>[4x]MSKK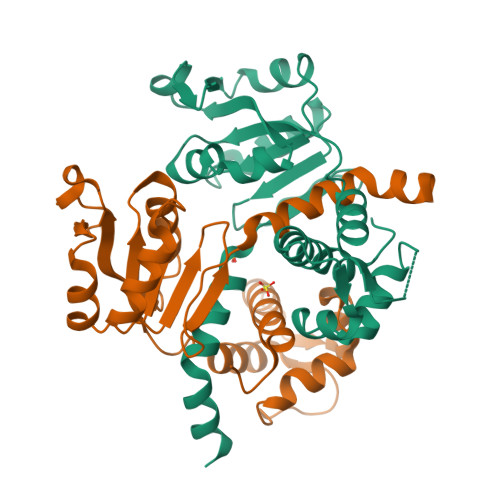TIVSMAVIRRLPRYHRYLEELLKNDVKRISSRELSEKMGVTASQIRQDLNNFGGFGQQGYGYNVEELYNNLTKILGLDKTYNTIIIGAGNLGQAIANYTSFEKSGFNLKGIFDINPRLFGLKIRDVEVMDVETVEDFIARNKIDIGILCIPKDNAQYTADRLVRAGIKAIWNFLPIDLKVPDDVILENVHLSDSLFTVSYRLNEEELFKKLKGETAKIDG Anaerobic ammonium oxidation (anammox) is a bacterial process in which ammonium and nitrite are combined into dinitrogen gas and water, yielding energy for the cell. As anammox bacteria express a large number of small c-type cytochromes, these have been proposed to perform the shuttling of electrons between the various parts of the metabolic machinery. Here, we present the structures and biochemical characterization of two of these proteins from the anammox model organism Kuenenia stuttgartiensis: Kustc0562 and highly homologous Kustc0563, which show relatively high transcription levels. Kustc0562 and Kustc0563 share 37% sequence identity after cleavage of the signal sequence and display a typical type-I cytochrome c fold.

Indeed, Kustc0563 was the first protein from an anammox organism to be purified from biomass and also the first to be heterologously expressed and characterized. In the crystal structure of Kustc0563, the heme iron is proximally coordinated by His47 and distally by Met91; in Kustc0562, the iron is proximally coordinated by the homologous His51, but the distal ligand is an imidazole molecule, presumably from the crystallization solution. Similar results were obtained when Kustc0563 was treated with imidazole, but this protein could be crystallized without it. Spectropotentiometry revealed that Kustc0562 and Kustc0563 have redox potentials of +244 and +268 mV versus standard hydrogen electrode (SHE), respectively. Importantly, however, the comparison of BtCytc with Kustc0563 shows that the latter protein supports hydroxylamine oxidation by KsHAO at a rate that is approximately 6 times higher (kcat = 48.4 s–1, Km = 13.9 μM). The simulations predict a preferential interaction surface between Kustc0563 and KsHAO. On Kustc0563, this involves a ring of negatively charged residues on the surface around the heme, in addition to several hydrophobic and two positively charged residues. The predicted interaction surface on HAO displays a pronounced positive charge, which would complement the equally pronounced negative charge on the predicted interaction surface on Kustc0563. Moreover, in the related Kustc0457/Kustc0458 complex, the typical 24-heme electron transport system of HAO-like Kustc0458 is extended from its heme 1 onward with the hemes of the complex partner Kustc0457.3 Interestingly, however, in our simulations, heme 3, which in KsHAO lies at the surface of the protein at the bottom of the concave surface between the protrusions, is consistently predicted to be part of the interaction surface with Kustc0563. This opens up the possibility that in the interaction between KsHAO and Kustc0563, heme 3 is the outlet for electrons rather than heme 1.

> SNIDGMKLYLQHCKTCHGVDGNPTDLGEGLGARKFADAEWQAKTSDERIIEQINEGTPEMMMPFKEKLTPEEVKALVPVVRGFKK>GSAAAQDMVSPPPPIADEPLTVNTGIYLIECYSLDDKAETFKVNAFLSLSWKDRRLAFDPVRSGVRVKTYEPEAIWIPEIRFVNVENARDADVVDISVSPDGTVQYLERFSARVLSPLDFRRYPFDSQTLHIYLIVRSVDTRNIVLAVDLEKVGKNDDVFLTGWDIESFTAVVKPANFALEDRLESKLDYQLRISRQYFSYIPNIILPMLFILFISWTAFWSTSYEANVTLVVSTLIAHIFFNILVETNLPKTPYMTYTGAIIFMIYLFYFVAVIEVTVQHYLKVESQPARAASITRASRIAF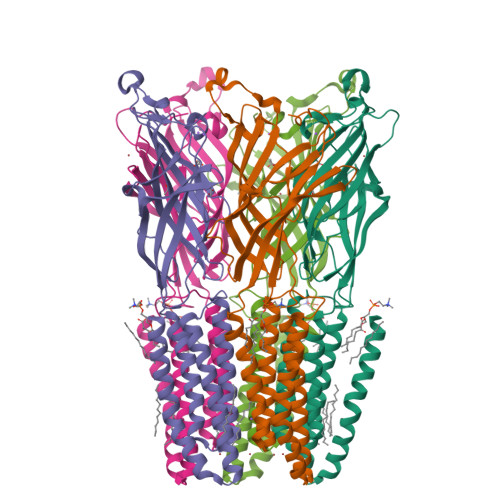PVVFLLANIILAFLFFG[5x]(2S)-2-[(1S,2R)-1-carboxy-2-hydroxypropyl]-4-{[(3S,5S)-5-(dimethylcarbamoyl)pyrrolidin-3-yl]sulfanyl}-3-methyl-2H-pyrrole-5-carboxylic 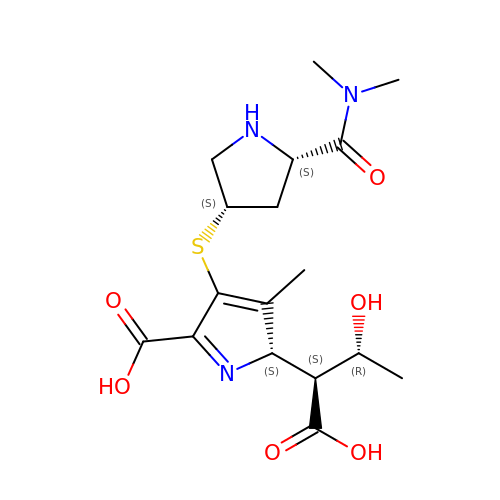acid | C17 H25 N3 O6 S | AGLQJULLKPLWOW-YBXAARCKSA-N> 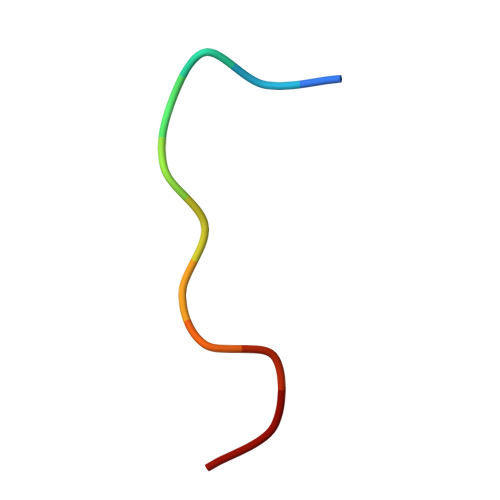FSIVGSLPRDC>MTNVFESSPLFLRILLAVLIILLFFYFIFLNYREYKNNNQVKQLNAKVRSLITGHYTDKLKVEDNSDLSELVNNVNDLSEVFRLTHENLAQEKNRLTSILSYMTDGVLATDRSGKITVINDMAQKQLNVTREQALECNILDILDDDSYTYNDLITKTPEIVLTRRDEYDEFITLRIRFALNRRESGFISGLIAVLHDATEQEKEERERRLFVSNVSHELRTPLTSVKSYLEALDDGALTESVAPSFIKVSLDETNRMMRMITDLLSLSRIDNQTSHLDVELTNFTAFMNYILDRFDQIQSQQSTNKVYEIIRDYPDKSVWIEIDTDKMTQVIDNILNNAIKYSPDGGKVTITMQTTDTQLILSISDQGLGIPKKDLPLIFDRFYRVDKARSRAQGGTGLGLAIAKEIVKQHKGFIWANSEEGEGSTFTIVLPYENDNDAIDEWEEDEDES[2x]

Bacteria respond to transient living environments through transmembrane-integrated sensor histidine kinases (SKs), which act in concert with their intracellular cognate response regulators (RRs) to elicit necessary adaptive responses that are critical for their survival and virulence. The SKs and RRs have evolved into a two-component signal transduction system (TCS), whereby stimulation of the SK autophosphorylates at a conserved histidine residue to initiate a signaling cascade. The VicRK in S. mutans, which is an important pathogen in caries etiology, regulates acid production and tolerance conducive to dental caries, including proton expulsion (F1F0-ATPase). In addition, VicK has one HAMP domain and one PAS domain.

In this study, we report the crystal structure of the entire intracellular portion of VicK (aa 31–450), which comprises an SK dimer with one signal transducer, one signal sensor, and one intact kinase domain. VicK crystals diffracted slightly better than 3 Å; however, because of strong anisotropy, the final structure was refined up to only 3.3 Å. The overall structure of VicK comprises a dimer in the shape of a long slim rod. In addition, the HAMP, PAS, and DHp domains are organized as dimers, which are connected by long, straight coiled-coils of helices α2 and α6. The VicK HAMP domain appears to be a stable four-helix coiled-coil with classical knobs-into-holes interactions, wherein three pairs of hydrophobic residues from helix α2 form a central hydrophobic core with knobs-to-knobs packing, and it is unlikely that structural alternations of the HAMP domain play a central role in signal transmission. The VicK PAS domains form a unique dimer, which is mediated by a leucine-zipper. The dimeric architecture of these domains looks like a butterfly, wherein the DHp domain (aa 199–269) is a four-helix bundle of helices α6 and α7 with a phosphoryl receptor histidine located in the middle. Interestingly, the two monomers of the DHp domain bear an asymmetric fold. However, the upper parts of helices α6 and α7 are remarkably different, wherein helix α6 bends ∼25° at Pro222 toward the central DHp axis and α7 moves ∼11° away in the opposite direction to avoid a possible clash. Although the overall conformation of each CA domain in VicK is the same, their positions relative to the DHp domain show dramatic differences, which generates an asymmetrical ATPase dimer.> MNIFRLTGDLSHLAAIIILLLKIWKSRSCAGISGKSQLLFALVFTTRYLDLFTSFISLYNTSMKLIYIACSYATVYLIYMKFKATYDGNHDTFRVEFLIVPVGGLSFLVNHDFSPLEILWTFSIYLESVAILPQLFMISKTGEAETITTHYLFFLGLYRALYLVNWIWRYYFEGFFDLIAVVAGVVQTVLYCDFFYLYVTKVLKGKKLSLPAGENLYFQ;> AERDEL

In the archetypal KDEL-retrieval system, a seven-transmembrane receptor captures escaped ER luminal proteins carrying a C-terminal KDEL or variant tetrapeptide sequence in the mildly acidic pH of the Golgi. Signal binding to a luminal cavity in the receptor triggers a conformational change in its cytoplasmic face, exposing a lysine motif recognised by the COP I coat complex. Hence, the KDEL receptor cycles between the ER and Golgi capturing escaped ER proteins in a dynamic retrieval process. Our previous work has shown the KDEL receptor has a transporter-like architecture and undergoes pH-dependent closure around cognate retrieval signals.

We then determined structures for chicken KDELR2 bound to HDEL and RDEL signals. These structures with TAEHDEL and TAERDEL peptides have resolutions of 2.24 and 2.31 Å, respectively. In both instances the overall structure of the receptor is similar to our previous complex with the TAEKDEL peptide, with a root mean square deviation (R.M.S.D.) of 0.223 and 0.153 Å over 200 Cα atoms for the HDEL and RDEL structures, respectively. Both HDEL and RDEL peptides are bound in a vertical orientation with respect to the membrane, with the side chains clearly resolved in the electron density map. Superimposing the three peptides reveals little movement of the peptide at the −1 and −2 positions when bound to the receptor. For RDEL, we observe slight movement of the backbone Cα atom of the peptide to accommodate the larger arginine side chain, resulting in a minor repositioning of the glutamate at the −3 position in the receptor. Nonetheless, the position of the positive charge at the −4 position on all three peptides is identical relative to E117 and W120 within the receptor, supporting the view that a salt bridge is formed with E117 on TM5. For RDEL, the arginine side chain sits in the same position as the amine group of KDEL and could thus interact with W120 via a cation-π interaction and E117 via a classical salt bridge interaction. We therefore conclude that both E117 and W120 play a role in retrieval signal binding, and the only major difference between HDEL, RDEL, and KDEL is the precise nature of the interaction with W120 indicating that this may be a critical residue to explain the differences in affinity.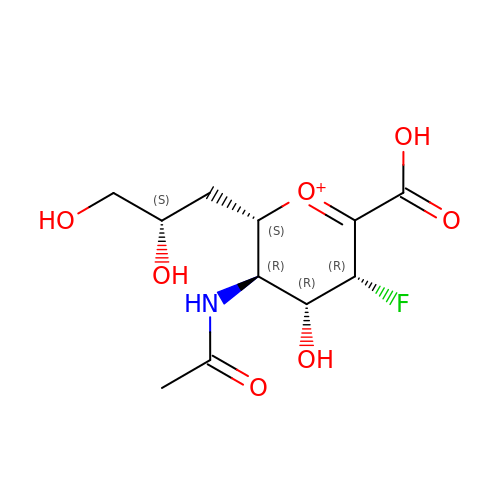(2~{S},3~{R},4~{R},5~{R})-3-acetamido-2-[(2~{S})-2,3-bis(oxidanyl)propyl]-5-fluoranyl-4-oxidanyl-2,3,4,5-tetrahydropyran-1-ium-6-carboxylic acid | C11 H17 F N O7 | DFROFKMCNZKOFD-PQFOHKHZSA-O> GAGCAGACTTGACGAGACTCA;> TCG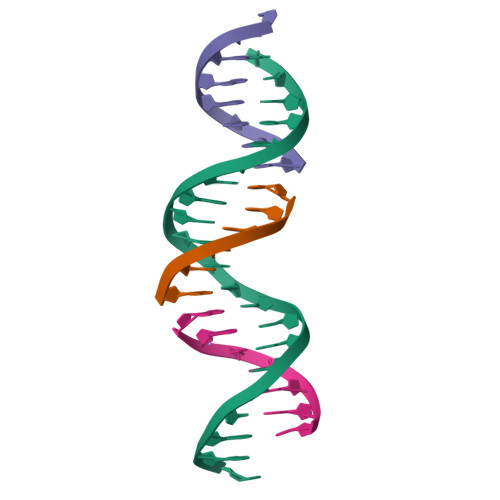TCA;> TCTGAGTC;> AGTCTGC>[2x]MSKLEAILSQEVEAEIQALLQEAEAKAEAVKREAEEKAKALLQARER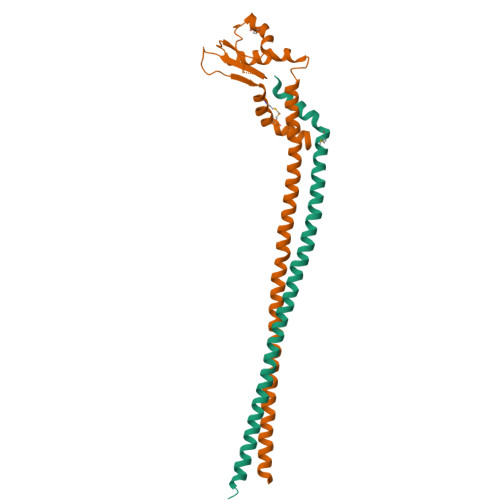ALEAQYRAALRRAESAGELLVATARTQARGEVLEEVRRRVREALEALPQKPEWPEVVRKLALEALEALPGAKALVANPEDLPHLEAMARERGVELQAEPALRLGVRAVGAEGKTQVENSLLARMDRAWDAMSSKVAQALWG;>GGGLGLIKSLAEKEKQLLERLEAAKKEAEERVKRAEAEAKALLEEAEAKAKALEAQYRERERAETEALLARYRERAEAEAKAVREKAMARLDEAVALVLKEVLP[2x]>[4x]GAMDIVVNDDLSCRFLEGFNTRDALCKKISMNTCDEGDPFFVADLGDIVRKHETWKKCLPRVTPFYAVKCNDDWRVLGTLAALGTGFDCASNTEIQRVRGIGVPPEKIIYANPCK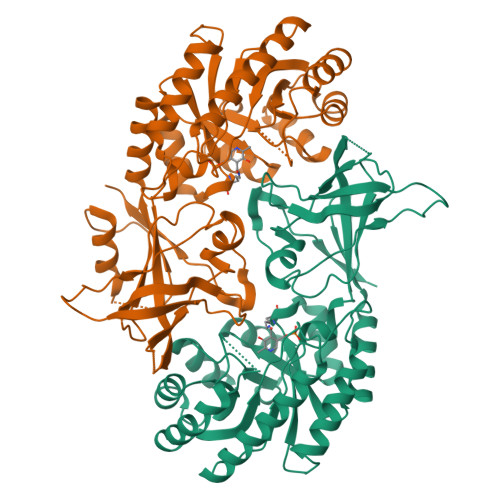QISHIRYARDSGVDVMTFDCVDELEKVAKTHPKAKMVLRISTDDSLARCRLSVKFGAKVEDCRFILEQAKKLNIDVTGVSFHVGSGSTDASTFAQAISDSRFVFDMGTELGFNMHILDIGGGFPGTRDAPLKFEEIAGVINNALEKHFPPDLKLTIVAEPGRYYVASAFTLAVNVIAKAVTPGVQTDVGAHAESNAQSFMYYVNDGVYGSFNCILYDHAVVRPLPQREPIPNEKLYPSSVWGPTCDGLDQIVERYYLPEMQVGEWLLFEDMGAYTVVGTSSFNGFQSPTIYYVVSGLPDHVVRELKSQKS>MEIVEYPDPILRAKNKRIDIFDENLKNLVDAMFDVMYKTDMIGLSAPQVGLNVQLMVFNPAGEPGEGKEIVLVNPKIKKYSDKLVPFDEGCLSFPGIYAEVVRPQSVKIDARDITGERFSISLSRLPARIFQHEYDHLEGVLFFDRMTDQVLDSIREELEALEKKYEEKTGLPSPERVEARQKRKAGVGFGKR[4x]

Here, we explore the precise structural inhibitory mechanism of actinonin, which is a slow, tight-binding inhibitor of peptide deformylase (PDF), a metal cation-dependent enzyme. PDF is the first enzyme in the N-terminal methionine excision pathway, an essential and ubiquitous process that contributes to the diversity of N-terminal amino acids. The function of the active-site metal is to activate the reactive water molecule involved in peptide hydrolysis. Actinonin is a natural product with antibiotic activity that inhibits PDF by mimicking the structure of its natural substrates (nascent peptide chains starting with Fo-Met-Aaa, where Fo is a formyl group and Aaa is any amino acid) in their transition state.

For all variants of position G41, addition of actinonin to the crystal induced a closure of the protein within the crystal. Nevertheless, as expected from in silico graphic modeling followed by energy minimization, the occurrence of a bulky side chain at position 41 prevented the completion of the closure in the presence of the ligand and, hence, the formation of the hydrogen bond between the backbone nitrogen of Ile42 and actinonin. m of the complex of the variants with actinonin compared to WT as measured by DSC. Remarkably, both S and O forms of the G41M apo-structures in the asymmetric unit of the crystal yielded a unique intermediary structure (“I” state) upon actinonin binding (r.m.s.d. between the molecules is <0.25 Å; see also Figure 2B, zone “I”). In this case, it is likely that the induced-fit mechanism drives the equilibrium by capturing only the O population and closing it to an intermediary step, thus depleting the pool of O conformers that is shifted sequentially back from the remaining pool of S conformers and allows the complete binding of actinonin to the enzyme. In line with the rational design of the PDF mutants, the extent of the structural differences suggests that the underlying motions are dependent on the length of the side chain. Together, these data account for the reduced catalytic rate, as the hydrogen bond is strictly required for the substrate to be efficiently cleaved by PDFs. Thus, our study of the designed Gly41 mutant enzymes reveals that, in addition to the initial and final states observed for the WT enzyme, the conformations of the Gly41 variants correspond indeed to on-pathway intermediates, thus providing snapshots along the trajectory from the O to the C state of the enzyme. Progression to this closure involves intermediary states (“I”) similar to those observed with variants G41Q and G41M in the presence of actinonin. Therefore, from both structural and kinetic analyses, each substitution most likely reproduces intermediates along the pathway that lead to the closure of PDF around its substrate.>[4x]GPGIQVKALYDYDAQTGDELTFKEGDTIIVHQKDP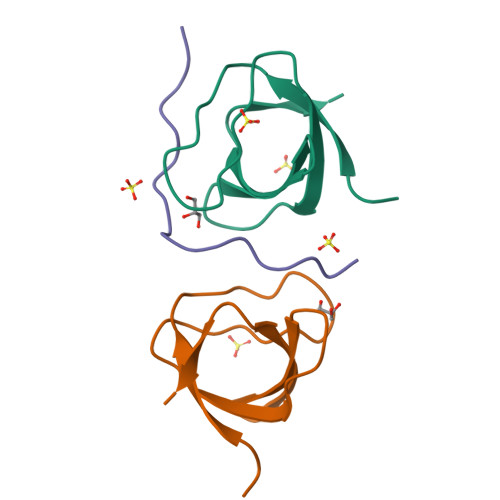AGWWEGELNGKRGWVPANYVQDI;>AKPVPPPRGAKPAPPPRT[2x]> SNAMTKSRFFSDVAETSSFVFAVAGADDEVVLETIRLALKQKLGKFLLFGKKEDKTLTANESVTWIQTDTAEAAAQGAILAVKNKEADILVKGFIPTATLMHHVLKKENGLRTDQLLSQIAIFDIPTYHKPLLITDCAMNVAPKTKEKIAITENALAVAHQIGITNPKIALLSAVEEVTAKMPSTLEAQEVVQHFGNQISVSGPLALDVAISKEAALHKGITDSSAGEADILIAPNIETGNALYKSLVYFAGAKVGSAVVGAKVPIVISSRNDSPENKLASFILT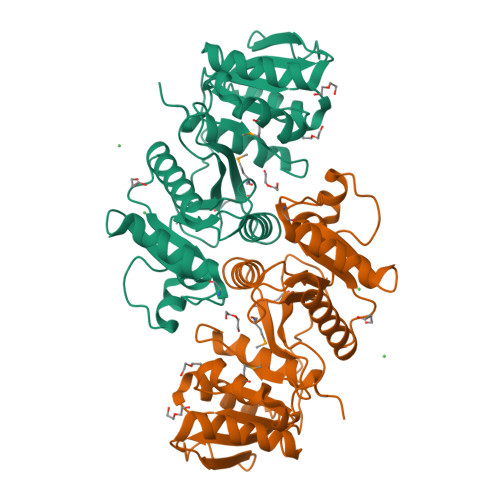VRLVEK> FSGSE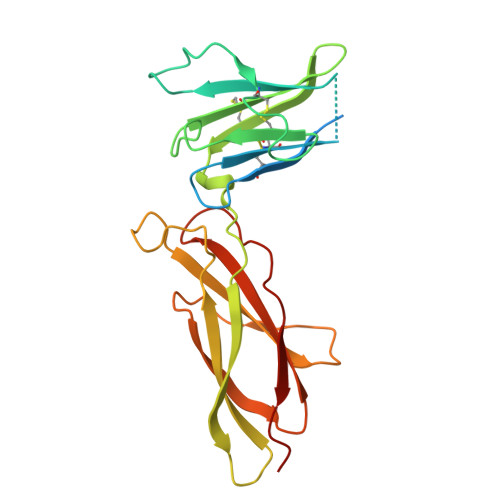ATAAILSRAPWSLQSVNPGLKTNSSKEPKFTKCRSPERETFSCHWTDEVHHGTKNLGPIQLFYTRRNTQEWTQEWKECPDYVSAGENSCYFNSSFTSIWIPYCIKLTSNGGTVDEKCFSVDEIVQPDPPIALNWTLLNVSLTGIHADIQVRWEAPRNADIQKGWMVLEYELQYKEVNETKWKMMDPILTTSVPVYSLKVDKEYEVRVRSKQRNSGNYGEFSEVLYVTLPQMSQ>MHHHHHHAMGTLTPHKTISFGSLTIDPVNRQVMLGGENVALSTADFDMLWELATHAGQIMDRDALLKNLRGVTYDGMDRSVDVAISRLRKKLLDNATEPYRIKTVRNKGYLFAPHAWDN[2x]

The RstB/RstA system is a ubiquitous TCS composed of the membrane-associated histidine kinase RstB and its cognate response regulator RstA. K. pneumoniae RstA (kpRstA) contains an N-terminal receiver domain (RD, residues 1–119) and a C-terminal DNA-binding domain (DBD, residues 131–236), with an overall sequence identity of 79% compared to RstA from E. coli and S. enterica serovar Typhimurium. As a member of the OmpR/PhoB subfamily, phosphorylation of the conserved Asp in the RD is believed to result in dimerization of the domain through a conserved α4–β5–α5 region, accompanied by the binding of the DBD to cognate sequences in the promoter region of RstA-regulated genes. Genomic systematic evolution of ligands by exponential enrichment (SELEX) experiments in E. coli have shown that RstA binds to the consensus sequence TACATNTNGTTACA with tandem TACA recognition sites.

The crystal structure of kpRstA DBD/DNA-23 consists of two protein molecules and one 23-bp DNA per asymmetric unit. The two DBDs bind on the same side of the DNA in a head-to-tail fashion and the electrostatic potential surface of the protein dimer forms a long and continuous positively charged region for DNA binding. The α3 recognition helix is docked into the major groove of the DNA and forms numerous interactions with the RstA box. The C-terminal β-hairpin also makes contact with the DNA, mostly close to the phosphate backbone. Unlike the bent DNA conformation observed for the PhoB DBD/DNA complex, the DNA-23 in kpRstA DBD/DNA-23 complex only displayed slight bending (∼10°). The two DNA-bound DBDs interact with each other with a buried surface area of 362 Å2 per monomer at the protein–protein interface. The interface mostly consists of β4 and β5 of the upstream DBD (bound to the 5′ half-site of the coding strand) on one end and the two loops between β2–β3 and β3–α1 of the downstream DBD (bound to the 3′ half-site of the coding strand) on the other end. The two kpRstA DBDs within an asymmetric unit bind to the DNA with similar contacts, with contact surfaces of 882 Å2 between DNA and protein and 899 Å2 for the upstream and downstream protomers, respectively. Specific interactions between the α3 recognition helix residues and DNA, which include Val203-T6, Arg207-G5, Arg199-G17′ and Arg199-T16′, provide the basis for sequence specificity. Noticeably, the α3–β4 loop swings ∼90° towards the template strand of the DNA in the complex, which results in Ala216 interacting with the ribose part of G17′.>[2x]AHHHHHHPCCSNPCQNRGECMSTGFDQYKCDCTRTGFYGENCTTPEFLTRIKLLLKPTPNTVHYILTHFKGVWNIVNNIPFLRSLIMKYVLTSRSYLIDSPPTYNVHYGYKSWEAFSNLSYYTRALPPVADDCPTPMGVKGNKELPDSKEVLEKVLL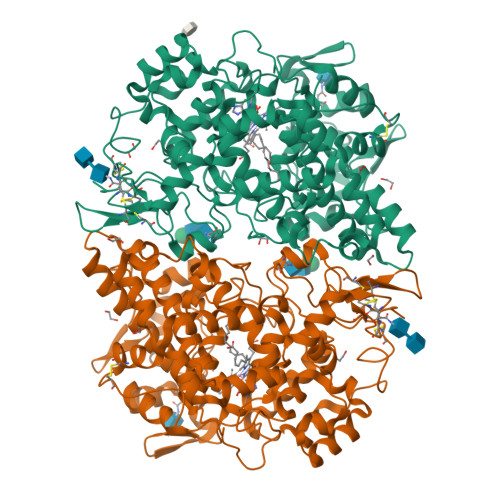RREFIPDPQGSNMMFAFFAQHFTHQFFKTDHKRGPGFTRGLGHGVDLNHIYGETLDRQHKLRLFKDGKLKYQVIGGEVYPPTVKDTQVEMIYPPHIPENLQFAVGQEVFGLVPGLMMYATIWLREHNRVCDILKQEHPEWGDEQLFQTSRLILIGETIKIVIEDYVQHLSGYHFKLKFDPELLFNQQFQYQNRIASEFNTLYHWHPLLPDTFNIEDQEYSFKQFLYNNSILLEHGLTQFVESFTRQIAGRVAGGRNVPIAVQAVAKASIDQSREMKYQSLNEYRKRFSLKPYTSFEELTGEKEMAAELKALYSDIDVMELYPALLVEKPHPDAIFGETMVELGAPFSLKGLMGNPICSPQYWKPSTFGGEVGFKIINTASIQSLICNNVKGCPFTSFNVQDPQPTKTATINASASHSRLDDINPTVLIKRRSTEL> A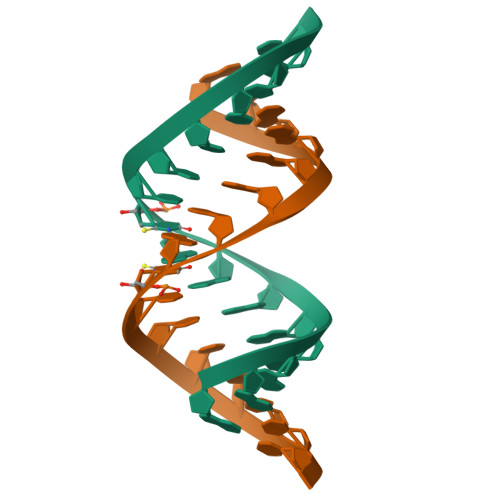GAGAAGAUCUUCUCU> MADLQHIKHMRTAVRLARYALDHDETPVACIFVHTPTGQVMAYGMNDTNKSLTGVAHAEFMGIDQIKAMLGSRGVVDVFKDITLYVTVEPCIMC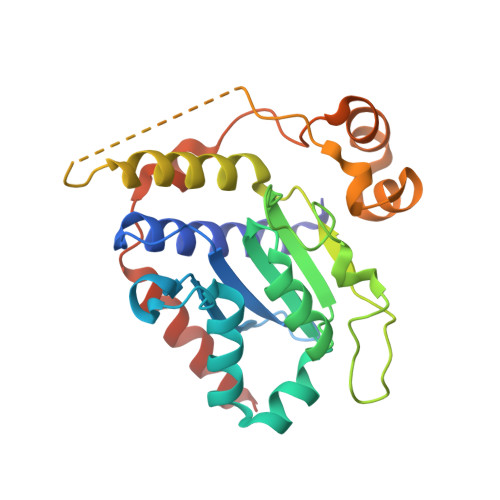ASALKQLDIGKVVFGCGNERFGGNGTVLSVNHDTCTLVPKNNSAAGYESIPGILRKEAIMLLRYFYVRQNERAPKPRSKSDRVLDKNTFPPMEWSKYLNEEAFIETFGDDYRTCFANKVDLSSNSVDWDLIDSHQDNIIQELEEQCKMFKFNVHKKSKV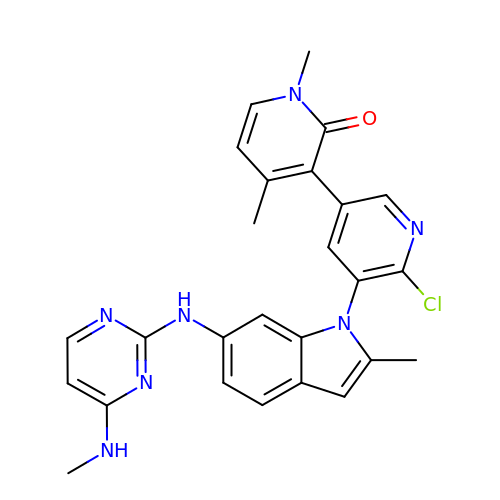6'-chloro-1,4-dimethyl-5'-(2-methyl-6-{[4-(methylamino)pyrimidin-2-yl]amino}-1H-indol-1-yl)-3,3'-bipyridin-2(1H)-one | C26 H24 Cl N7 O | UFLRBTMJLDXXGQ-UHFFFAOYSA-N> KETAAAKFERQHMDSSTSAASSSNYCNQMMKSRNLTKDRCKPVNTFVHESLADVQAVCSQKNVACKNGQ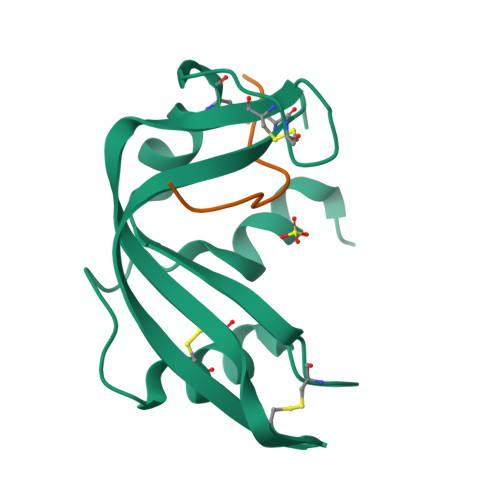TNCYQSYSTMSITDCRETGSSKYPNCAYKTTQANKHIIVACEGN;> PYVPVHFNASV>[2x]AAPLAATASKFLGCAYGAQQAPGFAQYWNKLTPENGGK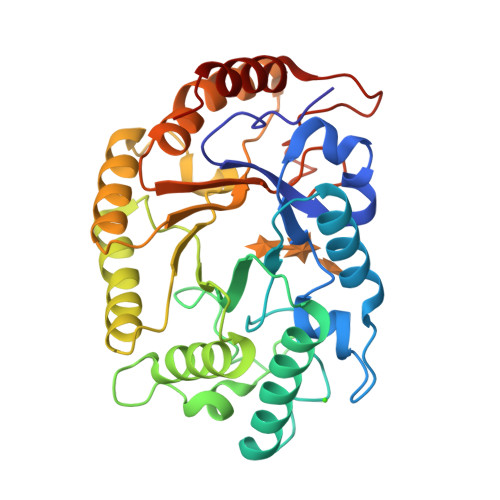WGSVEAVRDQMDWSTLDAAYRFAQANQMPFQMHVMVWGNQQPEWIKTLRPAEQRREIEQWFAAVAQRYPDIALLEVVNEPLNDPPSKADTGGGNYLQALGGNGDSGWEWVLQSFRLARRHFPHTKLMINDYSITSSAQATQKYLQIVRLLQRENLVDAIGVQEHAFETTPEVAVSVHRDNLDALAATGLPIYITEFDLDGPTDAQQLADYKRVFPVFWEHPAVHGITLWGFRPGLWRDKEAAYLIRADGTERPALTWLRDYVAAHPG>[2x]MGGEIITLQAGQCGNHVGKFLWSQLAKEHAIGTDGLSQLPDSSTERDDDTKPFFRENSRNKFTPRAIMMDSEPSVIADVENTFRGFFDPRNTWVASDGASAGNSWANGYDIGTRNQDDILNKIDKEIDSTDNFEGFQLLHSVAGGTGSGLGSNLLEALCDRYPKKILTTYSVFPARSSEVVVQSYNTILALRRLIEDSDATVVFDNASLLNISGKVFRNPNIDLQHTNQLISTIISSVTNSIRFPSYMYSSMSSIYSTLIPSPELHFLSPSFTPFTSDYIHDDIAHKGHSSYDVMLDLLDPSNSLVSTAMNNPTYFNVYNTIIGNVEPRQISRAMTKLQQRIKFPSWSSSAMHVNIGRRSPYLPLQPNENEVSGMMLSNMSTVVNVFENACNTFDKVFAKGAFLNNYNVGDLFQSMQNVQDEFAESREVVQSLMEDYVAAEQDSYLDDVLVDDENMVGELEEDLDADGDHKLV;> MELEPTLFGIIEALAPQLLSQSHLQTFVSDVVNLLRSSTKSATQLGPLIDFYKLQSLDSPETTIMWHKIEKFLDALFGIQNTDDMVKYLSVFQSLLPSNYRAKIVQKSSGLNMENLANHEHLLSPVRAPSIYTEASFENMDRFSERRS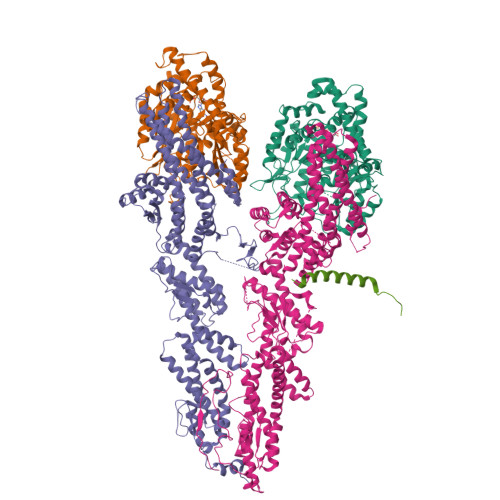MVSSPNRYVPSSTYSSVTLRQLSNPYYVNTIPEEDILKYVSYTLLATTSALFPFDHEQIQIPSKIPNFESGLLHLIFEAGLLYQSLGYKVEKFRMLNISPMKKALIIEISEELQNYTAFVNNLVSSGTVVSLKSLYREIYENIIRLRIYCRFTEHLEELSGDTFLIELNIFKSHGDLTIRKIATNLFNSMISLYYEYLMNWLTKGLLRATYGEFFIAENTDTNGTDDDFIYHIPIEFNQERVPAFIPKELAYKIFMIGKSYIFLEKYCKEVQWTNEFSKKYHVLYQSNSYRGISTNFFEIINDQYSEIVNHTNQILNQKFHYRDVVFALKNILLMGKSDFMDALIEKANDILATPSDSLPNYKLTRVLQEAVQLSSLRHLMNSPRNSSVINGLDARVLDLGHGSVGWDVFTLDYILYPPLSLVLNVNRPFGRKEYLRIFNFLWRFKKNNYFYQKEMLKSNDIIRSFKKIRGYNPLIRDIINKLSRISILRTQFQQFNSKMESYYLNCIIEENFKEMTRKLQRTENKSQNQFDLIRLNNGTIELNGILTPKAEVLTKSSSSKPQKHAIEKTLNIDELESVHNTFLTNILSHKLFATNTSEISVGDYSGQPYPTSLVLLLNSVYEFVKVYCNLNDIGYEIFIKMNLNDHEASNGLLGKFNTNLKEIVSQYKNFKDRLYIFRADLKNDGDEELFLLSKSLR;> MEIKEVDDRAELLRYTNNIPLLGKLVNHQPLWSTNPKLKSFSLEKISAPDQRRVQEALVVKDLLNVLIGLEGTYIRYFNDYEPSDPETPIEFKIAKKMDPSFKTFSRRIVRYGKQYMILTRAYEKWSDTSFGMVLQRFAYEIRRFLEDVYLKTLVERLERDFNKVPNFSIRELEQIINETEVNKQMELLYNIYEEIFREIEERRTNQSSQEDFNNFMDSMKNESSLHLRLMVAFDTTVYPVPKGGAILKIFQQKILENLGDRSSVMFLKKLLNNISQDYCTMLYEWLTQGILNDPYQEFMTYDDLEGKTDNIFDTRDRAWDTQYFIRKDVLLRDCDSEEDKNLLFKMLRTGILLKVVRASLQIPTIPSNSSDITIQEINDFADLMEGSNLELYVDKCYSRANEIFLKLFFQGYDLINVLKHLQQIFLGYQSGHNVLKFLTKNMGELTKHYRNDNNANYDKLLQNFELERQSENPNNLMRQLLMIQFDTETLPQVLSHYLQIYPEVPENNSANDDSDPLMHANNFKNMNAILFDELSKERTGAYHGSNLELYTPKSAIYHLKFDINIPYPLNIIISRTCMIKYQIILRYQLVLQYHSRLLDETWMDLNKTPSWKYRGYSHTVKRRIVRATRVLHAKMNHFIKTIMEYFNQNVIDKEVYSLEKCYRNPTLAVAIQNELEGGLTNIMTNRCLSDLIPLQLQIFDIVYKFCKFIKSMRAKLCQLDPVLYEKHKSGMMKTLNEGYRTNNGGQEDVGYQEDAALELIQKLIEYISNASSIFRKCLINFTQELSTEKFDFYDSSSVDAAGIERVLYSIVPPRSASASSQR;> MDEASHLPNGSLKNMEFTPVGFIKSKRNTTQTQVVSPTKVPNANNGDENEGPVKKRQRRSIDDTIDSTRLFSEASQFDDSFPEIKANIPPSPRSGNVDKSRKRNLIDDLKKDVPMSQPLKEQEVREHQMKKERFDRALESKLLGKRHITYANSDISNKELYINEIKSLKHEIKELRKEKNDTLNNYDTLEEETDDLKNRLQALEKELDAKNKIVNSRKVD>[2x]MSRSKRDNNFYSVEIGDSTFTVLKRYQNLKPIGSG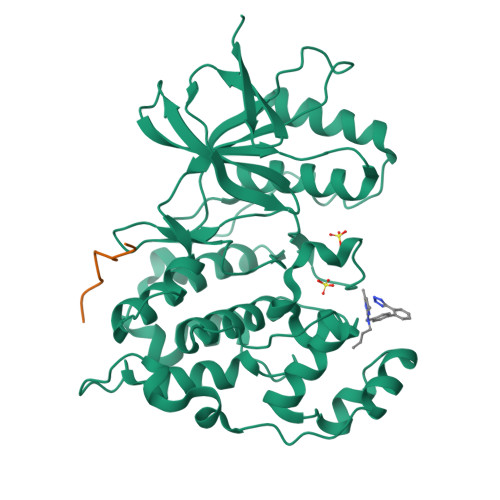AQGIVCAAYDAILERNVAIKKLSRPFQNQTHAKRAYRELVLMKCVNHKNIIGLLNVFTPQKSLEEFQDVYIVMELMDANLCQVIQMELDHERMSYLLYQMLCGIKHLHSAGIIHRDLKPSNIVVKSDCTLKILDFGLARTAGTSFMMEPEVVTRYYRAPEVILGMGYKENVDIWSVGCIMGEMVCHKILFPGRDYIDQWNKVIEQLGTPCPAFMKKLQPTVRNYVENRPKYAGYSFEKLFPDVLFPADSEHNKLKASQARDLLSKMLVIDASKRISVDEALQHPYINVWYDPSEAEAPPPKIPDKQLDEREHTIEEWKELIYKEVMDLEHHHHHH;>[2x]PKRPTTLNLF>MAANSTRRPIIAFMSDLGTTDDSVAQCKGLMYSICPDVTVVDVCHSMTPWDVEEGARYIVDLPRFFPEGTVFATTTYPATGTTTRSVAVRIKQAAKGGARGQWAGSGAGFERAEGSYIYIAPNNGLLTTVLEEHGYLEAYEVTSPKVIPEQPEPTFYGREMVAIPSAHLAAGF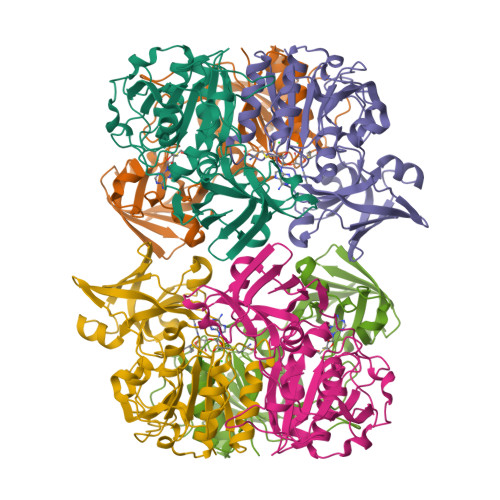PLSEVGRPLEDHEIVRFNRPAVEQDGEALVGVVSAIDHPFGNVWTNIHRTDLEKAGIGYGARLRLTLDGVLPFEAPLTPTFADAGEIGNIAIYLNSRGYLSIARNAASLAYPYHLKEGMSARVEAR[3x]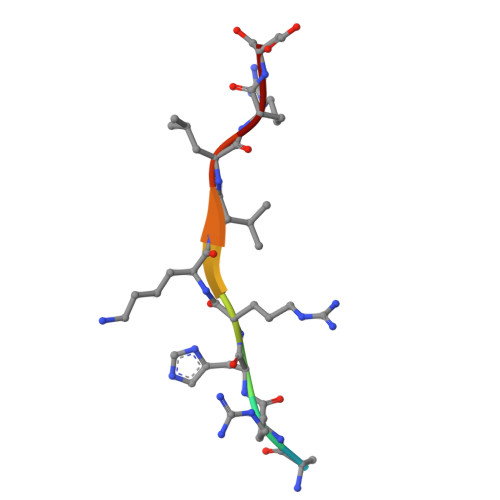> AKRHRKVLRD> 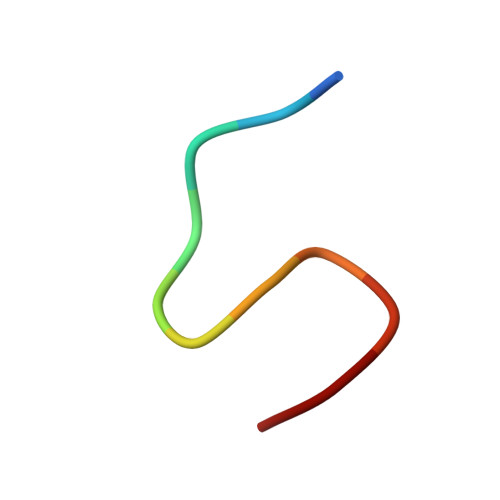TTLKFPSDWDD>MQEVTLTLHQFLPAQANVPKDVLDVWADNVEEASDGRIEIERYPSMQLGGTPPELMDQAIDGIADIVWTVVGYTPGRYPSTEVFELPFMVSDARAASYAYWKMFEEHMKDGEFADVKILGTWVHGPGMFHTNKPVAVPSDLEGMKIRGGSRLVNDLLTRVGAEPIGMPVPAISEALSKGVIDGTTIPWEVTSALKVPELVGNHTEFDGPALYNLTFV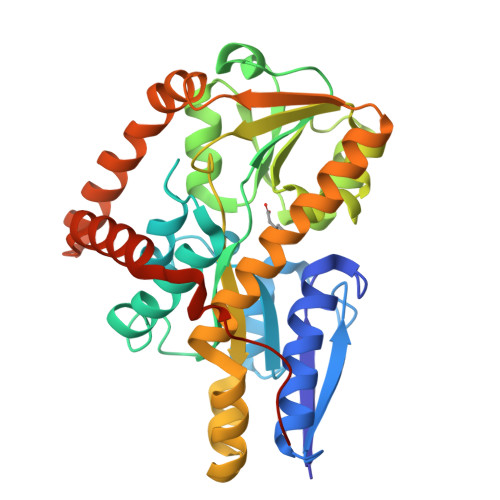LAMNKDAYESLPEDLQEVIDSQSGLAFSIFAGGTQADADGPARQIAVDRGNNIVTVSQEDAKAWDALVNPIYETWVAEMNDKGIDGQALIDEAKSLMEEYDPSMDTYGKAAALEHHHHHH[2x]Here, SAXS contrast data from an oligomeric protein and a protein–RNA complex are presented in the presence of iohexol and Gd-HPDO3A, two electron-rich molecules that are used in biomedical imaging and that belong to the families of iodinated and lanthanide-based complexes, respectively. For this, we applied two electron-rich medical contrast media, iohexol and Gd-HPDO3A, in SAXS experiments on a hexameric protein and a protein–RNA complex: protease 1 from Pyrococcus horikoshii and the aIF2:GDPNP:methionylated initiator tRNA complex from Saccharolobus solfataricus. Concentrated solutions of both media readily attained electron densities of 0.44 e− Å−3, equivalent to the upper range of typical protein densities.

Importantly, the experimental CMP (0.438 e− Å−3) was well within the range predicted from the protein sequence (0.420–0.443 e− Å−3) and the linearity of I(0)1/2 indicates that the oligomeric state of P1 was preserved at all Gd-HPDO3A concentrations. Altogether, the P1 data suggest that Gd-HPDO3A molecules are inert towards this protein and their presence (at up to molar concentrations) does not alter either the conformation of individual monomers or the overall oligomeric state and does not generate any appreciable solvation effects or specific interactions with the protein surface. The CMP thus determined (0.411 e− Å−3) was significantly lower than the range of values expected from the protein sequence (0.420–0.443 e− Å−3). Together, our data suggest that while preserving the oligomeric state of P1, iohexol preferentially interacts with the protein hexamer and/or changes the solvent properties close to its surface. In order to probe whether the specific binding of iohexol molecules can improve the quality of the SAXS fits, we generated P1 models with a single iohexol molecule bound in two distinct, opposite locations: either outside or inside the hexameric ring. P1 structures with an iohexol molecule modeled inside the ring improved the CRYSOL fit significantly, in particular in the shoulder region between 0.1 and 0.15 Å−1 (92 mM iohexol data), while the model with an iohexol molecule placed outside the ring decreased the quality of the fit. In parallel, the average electron density of the P1 hydration shell decreases by 10–20% with respect to the bulk at the highest (618 mM) iohexol concentrations.

>[6x]MKVLFLTANEFEDVELIYPYHRLKEEGHEVYIASFERGTITGKHGYSVKVDLTFDKVNPEEFDALVLPGGRAPERVRLNEKAVSIARKMFSEGKPVASICHGPQILISAGVLRGRKGTSYPGIKDDMINAGVEWVDAEVVVDGNWVSSRVPADLYAWMREFVKLLK> K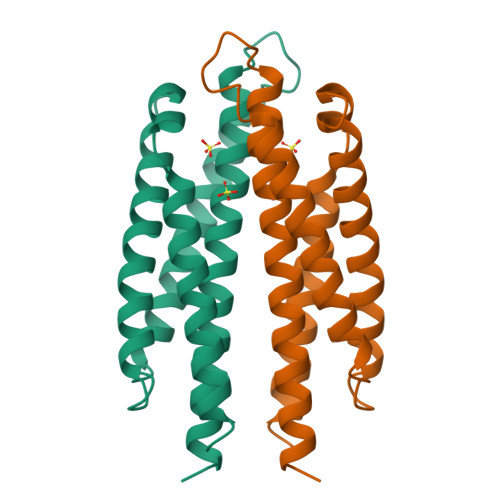SFVVSNQLREQQGELTSTWDLMLQTRINLSRSAVRMMMDSSNQQSNAKVELLDSARKTLAQAATHYKKFKSMAPLPEMVATSRNIDEKYKNYYTALTELIDYLDYGNTGAYFAQPTQGMQNAMGERFAQYALSSEKLYRDI> A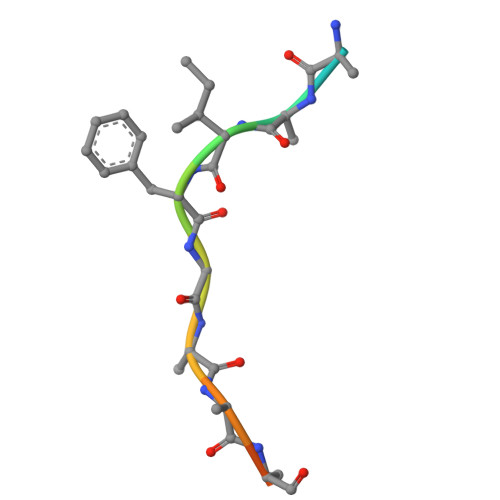EEEIFGEFEAKK>[2x]MGLAPLADGEKLYGKKGSEGTVTFTKAIGDNAFVEIKTGADTGFMNGCLGFSESIDGKNYWVAYVWQTKKSDTISIDMS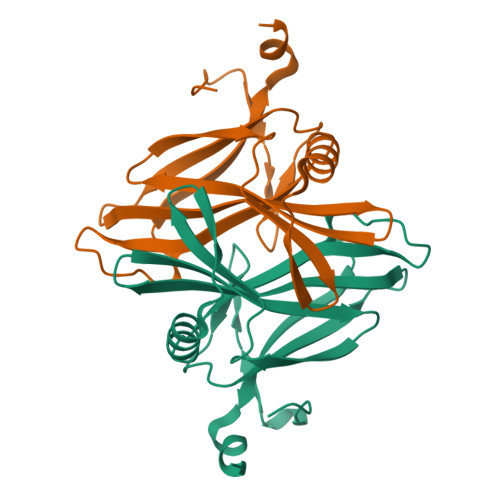SPVQIAEIIGTETQEVTDADTIKKLTDKIKTEKSALLQVWYASDKTGKQIDPADSASESIEVYIPSASADEALEHHHHHH> EGERKNNNKRWYFTREQLENSPSRRFGVDPDKELSYRQQAANLLQDMGQRLNVSQLTINTAIVYMHRFYMIQSFTRFPGNSVAPAALFLAAKVEGQPKKLEHVIKVAHTCLHPQESLPDTRSEAYLQQVQDLVILESIILQTLGFELTIDHPHTHVVKCTQLVRASKDLAQTSYFMATNSLHLTTFSLQYTPPVVACVCIHLACKWSNWEIPVSTDGKHWWEYVDATVTLELLDELTH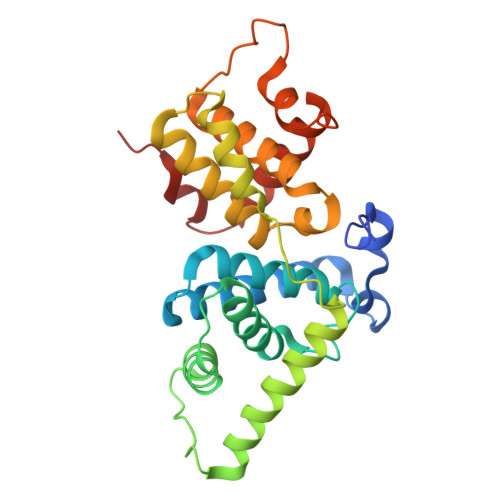ELLQILEKTPNRLKRIWNWR We sought to use our protocol to design a human transferrin receptor (hTfR) binding protein. hTfR transports transferrin (the major carrier of iron in the body) across the blood–brain barrier (BBB) via receptor mediated transcytosis, and this process has been exploited to deliver therapeutic payloads into the brain parenchyma that would otherwise be blocked by the BBB. We developed a computational design approach for designing binding proteins with beta sheets geometrically poised to pair with exposed beta strands in target proteins of interest. We targeted the region surrounding an edge strand located in the hTfR apical domain. This domain is distant from the transferrin binding site (which is important to avoid competitive binding) and is exposed and therefore suitable for beta sheet extension.

Combination of these enriched substitutions yielded higher affinity variants. The crystal structures of two increased affinity variants (2DS25.1 and 2DS25.5) in complex with hTfR were determined to be resolutions of 3.1 and 2.8 Å, respectively. The structures are virtually identical with an rmsd of 0.26 Å. In both cases, the design binds the Apical domain of hTfR using beta sheet extension and overall closely resembles the computational design model. The structure of 2DS25 superimposes closely on the computational model with an rmsd of 1.2 Å; this is notable as the fold is more complex than that of previous computationally designed binders. The majority of the mutants that improved binding map to the interface between hTfR and 2DS25 and likely optimize packing interactions and electrostatic contacts. Biolayer interferometry of five variants revealed KD’s ranging from 20 to 400 nM. Following injection of three Alexa488 labeled designs spanning two orders of magnitude in KD (2DS25 2 μM, 2DS25.3 200 nM, and 2DS25.5 20 nM) into the vascular channel, we observed transport of 2DS25.3 and 2DS25.5 into the CNS channel. Transport across the BBB was slightly higher for 2DS25.5 (Kd 20 nM) compared to 2DS25.3 (Kd 200 nM). An interface knockout (KO) variant of 2DS25 showed lower penetration into the CNS channel than 2DS25.3 and 2DS25.5, indicating the transport was specific.

>RLYWDDLKRKLSEKLDSTDFTSTIKLLNENSYVPREAGSQKDENLALYVENQFREFKLSKVWRDQHFVKIQVKDSAQNSVIIVDKNGRLVYLVENPGGYVAYSKAATVTGKLVHANFGTKKDFEDLYTPVNGSIVIVRAGKITFAEKVANAESLNAIGVLIYMDQTKFPIVNAELSFFGHAHLGTGDPYTPGFPSFNHTQFPPSRSSGLPNIPVQTISRAAAEKLFGNMEGDCPSDWKTDSTCRMVTSESKNVKLTVSNVLKEIKILNIFGVIKGFVEPDHYVVVGAQRDAWGPGAAKSGVGTALLLKLAQMFSDMVLKDGFQPSRSIIFASWSAGDFGSVGATEWLEGYLSSLHLKAFTYINLDKAVLGTSNFKVSASPLLYTLIEKTMQNVKHPVTGQFLYQDSNWASKVEKLTLDNAAFPFLAYSGIPAVSFCFCEDTDYPYLGTTMDTYKELIERIPELNKVARAAAEVAGQFVIKLTHDVELNLDYERYNSQLLSFVRDLNQYRADIKEMGLSLQWLYSARGDFFRATSRLTTDFGNAEKTDRFVMKKLNDRVMRVEYHFLSPYVSPKESPFRHVFWGSGSHTLPALLENLKLRKQNNGAFNETLFRNQLALATWTIQGAANALSGDVWDIDNEF[2x];>DEEEIQKAIEELLRKGVSEEEAAIIIVQRFNVAVVVVVQDERQGKHISEYIRRYIPEADVILFANLVVIKVETHELSTRVWEAAQKAY[2x]> G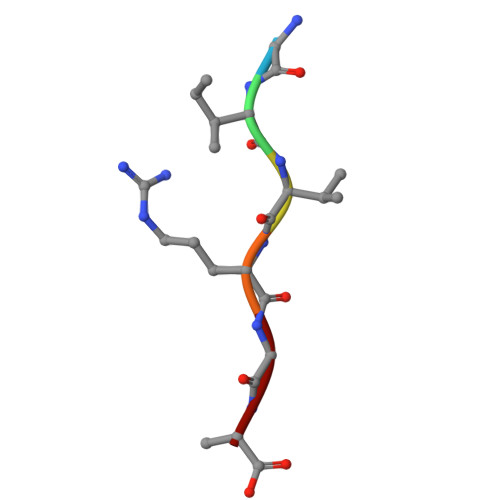IVRGA>DHVSSVRPNIFVGRVEGSAVYQKWYFEVTMDHIEKTTHMMPHLRIGWANTTGYVPYPGGGEKWGGNGVGDDLYSYGYDGAFLWSGGAKTGVNRTHAEEPYIRKGDVIGCALDLTVPIINFMFNGVRVTGSFTNFNLEGMFFPVISCSSKLSCRFLLGGEHGRLRYAAPPGYSPLVECLLPQQILSL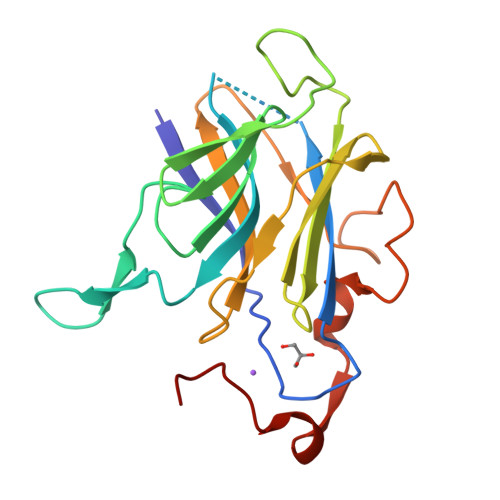EPCFCFGNL[2x]>PSVYDAAAQLTADVKKDLRDSWKVIGSDKKGNGVALMTTLFADNQETIGYFKRLGDVSQGMANDKLRGHSIVLMYALQNF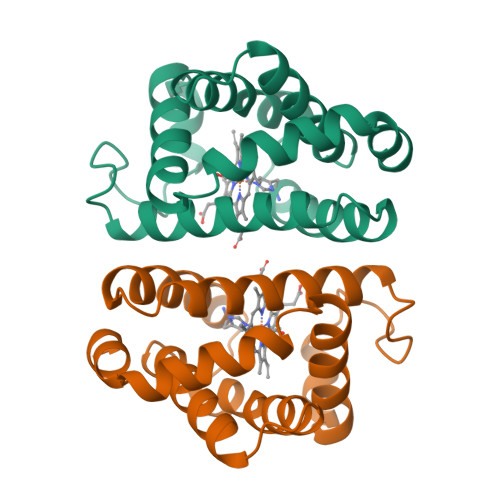IDQLDNPDDLVCVVEKFAVNHITRKISAAEFGKINGPIKKVLASKNFGDKYANAWAKLVAVVQAAL[2x]>CGCGAATTCGCG[6x]

Ridinilazole is a precision bisbenzimidazole antibiotic being developed to treat CDI and reduce unacceptably high rates of infection recurrence in patients. Unlike most currently used antibiotics which are natural-product based, ridinilazole is a symmetrical small molecule drug with a head-to-head bisbenzimidazole core. This structure is similar to nonsymmetrical, head-to-tail bisbenzimidazole Hoechst dyes, and ridinilazole has similar DNA-binding and intrinsic fluorescence properties. In combination, we present a conclusive array of data to indicate that ridinilazole exerts its antibiotic effect through a primary DNA binding mechanism which results in transcriptional dysregulation and C. difficile cell death.

The intrinsic fluorescence of ridinilazole was used to identify co-complex crystals through illumination of screening solutions with UV light; all four oligos yielded crystals of varying size and quality. dsOligo 1 (CGCGAATTCGCG) + ridinilazole produced rod-like crystals with blue fluorescence upon UV exposure, an X-ray diffraction data set was collected, and a resulting structure was determined to a resolution of 2.2 Å. Unexplained electron density was well described by the modeled ridinilazole molecule, confirming the compound binding location in the DNA minor groove. Ridinilazole was shown to adopt a curved snug fit typical of other minor groove binders, wrapping itself around the DNA with a dihedral angle of 34.5° between the two halves of the molecule. The model positions the symmetrical bisbenzimidazoles proximal to the core -AATT- of the double-stranded oligo with the bond connecting the symmetrical heterocycles positioned directly above the central -AT- pair. The central benzimidazoles both interact via their NH groups with neighboring nonpaired adenine and thymine bases; there are H-bonds from one NH to the adenine moiety of A6 (2.41 Å) and to the thymine moiety of T20 (2.33 Å), and from the other NH to the adenine moiety of A18 (2.43 Å) and the thymine moiety of T8 (2.29 Å). The four-position CH of the benzimidazoles H-bond with T19 (2.54 Å) and T7 (2.2 Å), respectively. On each of the terminal pyridyl groups, one 2-position CH interacts with a thymine carbonyl (T20 2.28 Å; T8 2.59 Å). The terminal pyridyl groups of ridinilazole bookend the complex through tight interactions with opposing deoxyribose groups on each strand. The overall structural positioning of ridinilazole was unambiguous and identical across the three molecules present in the unit cell. Most ridinilazole sequences identified in the footprinting contained a conserved AATT sequence which was coincident in the two oligonucleotides with greatest binding affinity and within the double-stranded oligo that yielded the ridinilazole:DNA structure.>QTDMSRKAFVFPKESDTSYVSLKAPLTKPLKAFTVCLHFYTELSSTRGYSIFSYATKRQDNEILIFWSKDIGYSFTVGGSEILFEVPEVTVAPVHICTSWESASGIVEFWVDGKPRVRKSLKKGYTVGAEASIILGQEQDSFGGNFEGSQSLVGDIGNVNMWDFVLSPDEINTIYLGGPFSPNVLNWRALKYEVQGEVFTK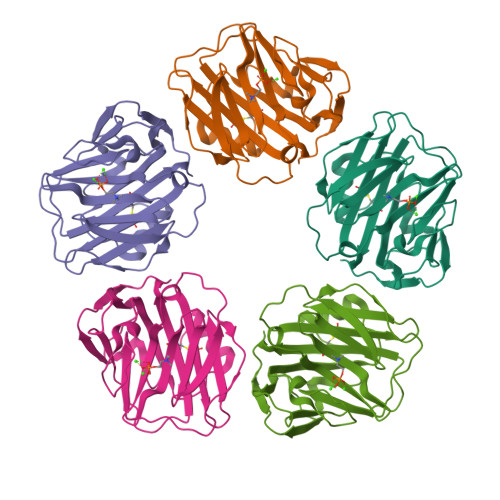PQLWP[5x]>MGGSTKLEEHLEGIVNIFHQYSVRKGHFDTLSKGELKQLLTKELANTIKNIKDKAVIDEIFQG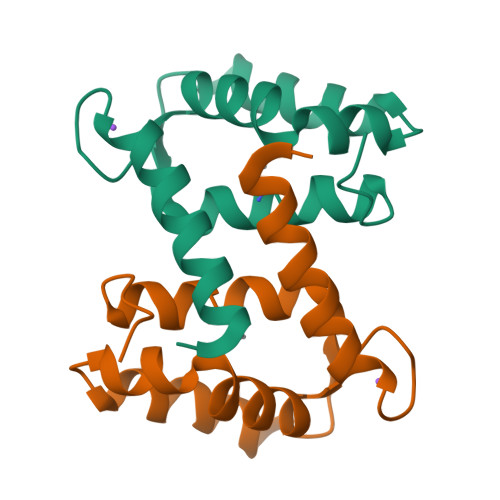LDANQDEQVDFQEFISMVAIALKAAHYHTHKE[2x]> MSWLTEEDIRRWESGTFYDSYRKLGAHPDDEGTWFCVWAPHADGVSVLGAFNDWNPEANPLERYGGGLWAGYVPGARPGHTYKYRIRHGFYQADKTDPYAFAMEPPTGSPIEGLASIITRLDYTWHDDEWMRRRKGPASLYEPVSIYEVHLGSWRHKRPGESFSYREIAEPLADYVQEMGFTHVELLPVMEHPYYGSWGYQVVGYYAPTFRYGSPQDLMYLIDYLHQRGIGVILDWVPSHFAADPQGLVFFDGTTLFEYDDPKMRYHPDWGTYVFDYNKPGVRNFLISNALFWLEKYHVDGLRVDAVASMLYRDYSRKEWTPNIFGGRENLEAIDFIKKFNETVYLHFPEAMTIAEESTAWPGVSAPTYNNGLGFLYKWNMGWMHDTLDYIQRDPIYRKYHHDELTFSLWYAFSEHYVLPLSHDEVVHGKGSLWGKMPGDDWQKAANLRLLFGHMWGHPGKKLLFMGGEFGQHHEWNHDTQLEWHLLDQPYHRGIQLWVCDLNHLYRTNPALWHDGPEGFEWIDFSDRDQSVICYLRKNAGRMLLFVLNFTPVPREHYRVGVPIGGPWHEVLNSDAVAYGGSGMGNFGRVEAVPESWHGRPFHLELTLPPLAALILEPEH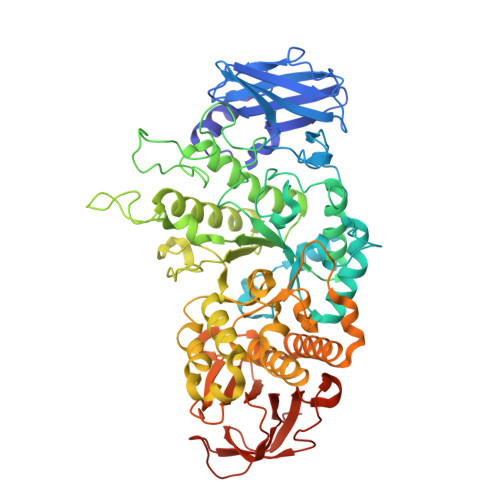G> QMNYEEVIKKYRGEENFDHAAYDWRLHSGVTPVKDQKNCGSCWAFSSIGSVESQYAIRKNKLITLSEQELVDCSFKNYGCNGGLINNAFEDMIELGGICPDGDYPYVSDA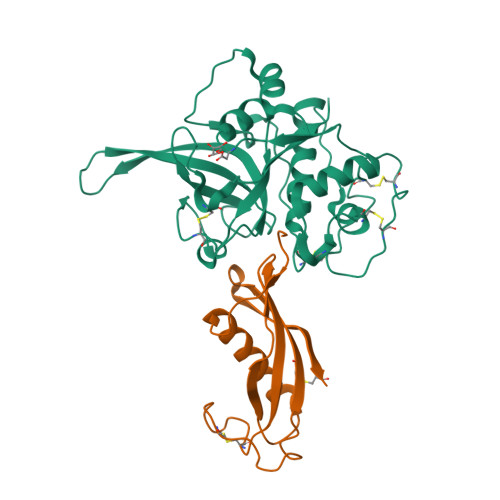PNLCNIDRCTEKYGIKNYLSVPDNKLKEALRFLGPISISVAVSDDFAFYKEGIFDGECGDQLNHAVMLVGFGMKEIVNPLTKKGEKHYYYIIKNSWGQQWGERGFINIETDESGLMRKCGLGTDAFIPLIE;> RLLGAPVPVDENDEGLQRALQFAMAEYNRASNDKYSSRVVRVISAKRQLVSGIKYILQVEIGRTTCPKSSGDLQSCEFHDEPEMAKYTTCTFVVYSIPWLNQIKLLESKCQ>[2x]MSLSDDPMASIKLLNLERENSAIAQYQSNIANLKTTLSSQETHLDSVSESLKSMRDIVLWGANGSLTDQDRSGMITELKSYRDSIESSFNAQDEEGHFLFSGTKTDTAALNKSSGA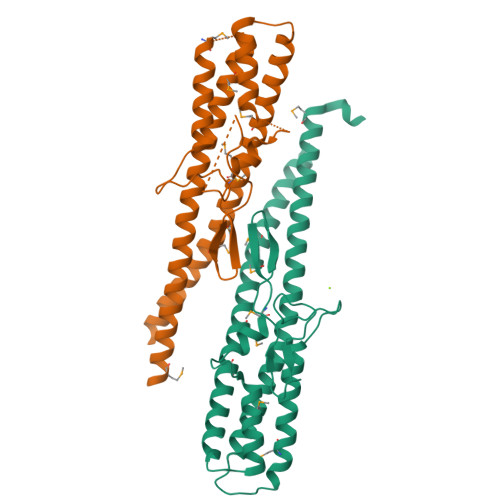YVVEGNSDVRVVTVAKGVTMDSNMTAQEILDIGGGKNVLNQIDALIAEFEKPSPNFQAEVDASLNAIDDTMANVLGAMTEIGGRHNNLDLMDGAHSENKLFVDKVSGDLSALDYGEGHHHHHH>SNAMEKVMATHFDYICIGGGSGGIASANRAAMYGAKVALIEAQDLGGTCVNVGCVPKKVMWHGAQIAEAMNLYAEDYGFDVDVKGFDWSKLVESRQAYIGRIHQSYDRVLGNNKVNVIKGFAKFVDEKTVEVNGEHYTADHILIAVGGRPTIPNIPGAEYGIDSNGFFDLAEQPKRVAVVGAGYIAVEIAGVLHALGTETHLFVRKESPLRSFDPMIIDTLVEVMEAEGPTLHTHSVPKEVVKEADGSLTLHLENGESQNVDQLIWAIGRHPATDAINLASTGVATNEKGYIKVDEYQETNVKGIYCVGDIMEGGIELTPVAVKAGRQLSERLFNNKP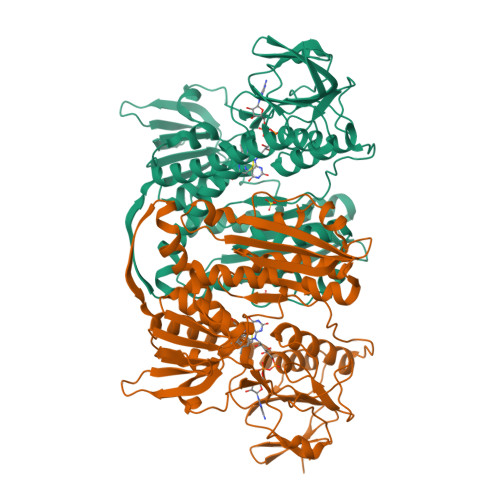NAKMDYDLVPTVVFSHPPIGTIGLTTQEAEEKYGKDNIKVYTSGFTAMYTAVTKHRQPCKMKLVCAGEEETVVGLHGIGFTVDEMIQGFGVAMKMGATKADFDSVVAIHPTGSEEFVTMR[4x]>MSVTEHKKQAPKEVRCKIVTISDTRTEETDKSGQLLHELLKEAGHKVTSYEIVKDDKESIQQAVLAGYHKEDVDVVLTNGGTGITKRDVTIEAVSALLDKEIVGFGELFRMISYLEDIGSSAMLSRAIGGTI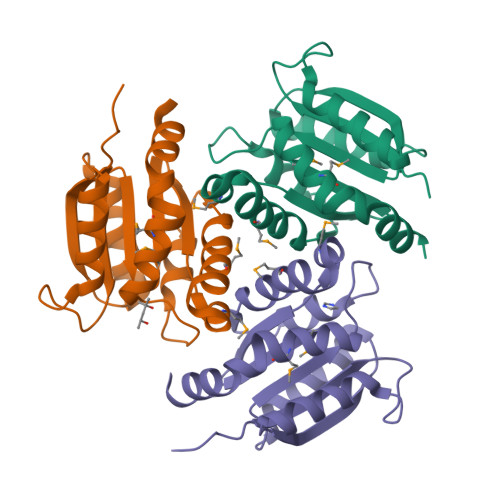GRKVVFSMPGSSGAVRLAMNKLILPELGHITFELHRQ[3x]3,3-dihydroxy-4-oxocyclohexa-1,5-diene-1-sulfonic 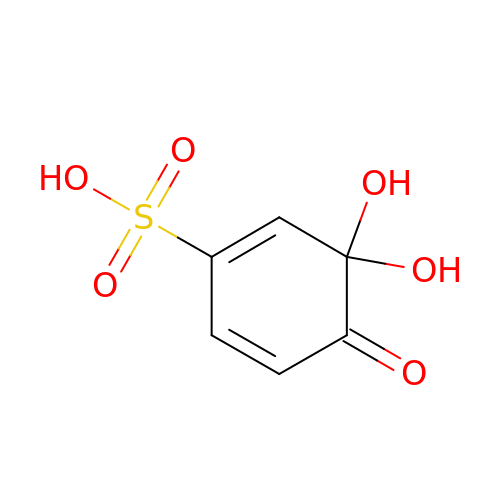acid | C6 H6 O6 S | JGCZOYLBGVHOFP-UHFFFAOYSA-N>MAMTLRDMDAVRPVNREAVDRHKARMRDEVRAFRLRELRAAQSLTQVQVAALAHIRQSRVSSIENGDIGSAQVNTLRKYVSALGGELDITVRLGDETFTLA[4x]

In the present study, we elucidated the crystal structure of Mycobacterium tuberculosis H37Rv HigA2 (hereafter referred to as MtHigA2), which contains an HTH motif. The HigA antitoxin represses the transcription of HigBA or forms a stable HigBA complex, thereby preventing the ribonuclease activity of the HigB toxin and the associated cytotoxic events. Structural studies of MtHigA2 confirmed that it has three regions: (i) a disordered N-terminus that is liable to cleavage, (ii) an α-helix bundle containing an HTH motif for DNA binding and (iii) a β-lid for dimerization. The antitoxin MtHigA2 has two binding partners: DNA and the toxin MtHigB2.

The crystal structure of MtHigA2 was determined from three distinct crystal forms. Form I belonged to space group P212121 and was determined to 2.0 Å resolution, form II packed in space group P43212 and was determined to 3.2 Å resolution, and form III was solved in space group P3121 to 3.4 Å resolution. Due to a lack of electron density at the N-terminus, ∼25 residues are undefined in each monomer despite the relatively high resolution. All dimers share the β-lid as their major dimeric interface, but the position of the α-helix bundle varies. When the different dimers are aligned based on a single HTH motif from one monomer, the corresponding motif in the dimer pair shows a different relative position. The flexibility in dimerization leads to drastic changes in the locations of positively charged residues on the HTH motif, including His54, Arg56 and Arg59. The greatest change in distance is that between the Nδ atoms of His54, which move by ∼7 Å [Figs. 1(c) and 1(d)]. To predict the physiological dimer, each form was submitted to the PISA server to calculate the strength of the dimer interface. Interestingly, all of the forms had similarly favourable dissociation energies (ΔG): −14, −15 and −17 kcal mol−1 for forms I, II and III, respectively. This suggests that the flexibility of the β-lid does not impact the formation of a stable dimer and is likely to contribute to function.PROPANAL | C3 H6 O | 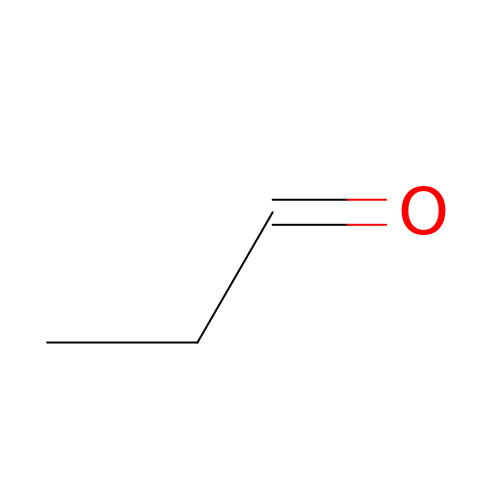NBBJYMSMWIIQGU-UHFFFAOYSA-N>GAGSMKSSTSKEKVCGENSRHIFNMILNSQRPQFDIK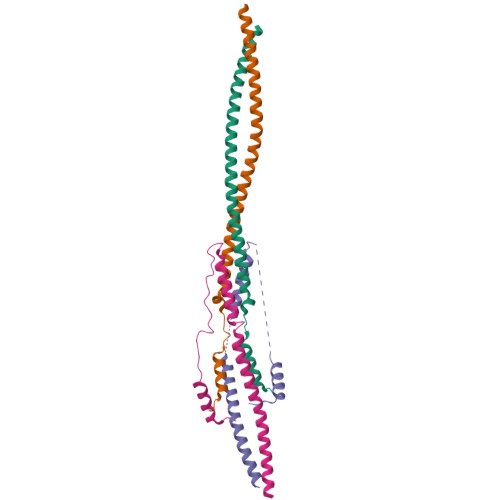DIGMFHLIDEIERLRKLWKDSEESKKRLNADMREAEEALAKARKKLAMFDIDVKDTQKHLRALMEENKALKLDLNVYETREKQLKDA[4x];>[4x]GHMGSSGGKQVERMPSERIPHSFFTQWNSELDGSVRMEDDGSREIPCPPTFCLTDCNDKDTVDSMYKYARKLSSLQNSSEEGPSSTLLTMIRQYMMEADYQRVEIARLKDSLNDKDEEIKKLRGFCSRYKRENA> GAMVKIIKKPKDVTALENATVAFEVSVSHDTVPVKWFHKSVEIKPSDKHRLVSERKVHKLMLQNISPSDAGEYTAVVGQLECKAKLFVETLHITKTMKNIEVPETKTASFECEVSHFNVPSMWLKNGVEIEMSEKFKIVVQGKLHQLIIMNTST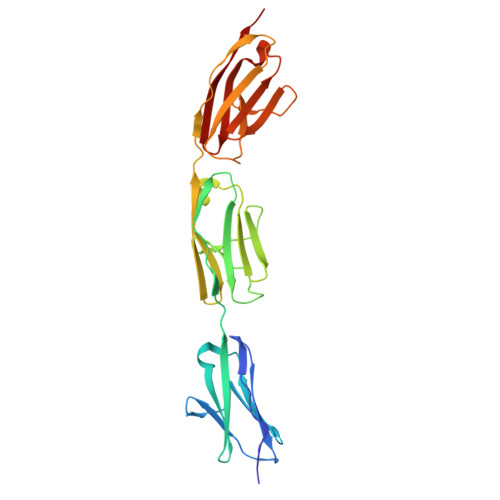EDSAEYTFVCGNDQVSATLTVTPIMITSMLKDINAEEKDTITFEVTVNYEGISYKWLKNGVEIKSTDKCQMRTKKLTHSLNIRNVHFGDAADYTFVAGKATSTATLYVVEA2-[8-(2~{H}-indazol-5-ylcarbonyl)-4-oxidanylidene-1-phenyl-1,3,8-triazaspiro[4.5]decan-3-yl]-~{N}-methyl-ethanamide 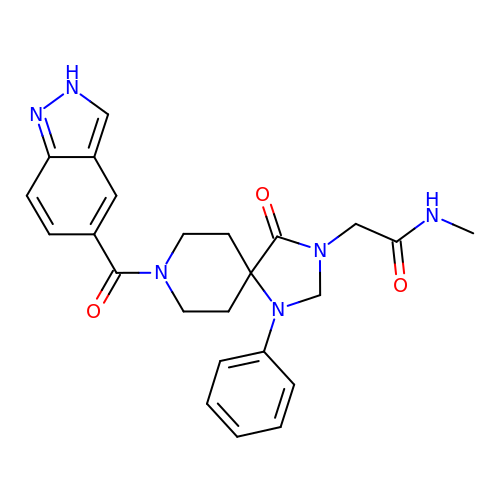| C24 H26 N6 O3 | QDMKAQVMVBLGFR-UHFFFAOYSA-N>GPLGSEKIEKDNAFAFDLLQTTRKHVTEANVFISPLSVSMALNMTLNGAAGVTADEMKTALRETGYTMEDINEYSHSLREALLKVDPSTTIGMANSIWYKQGELVKEPFILANRTHYDAEVKAVDFSSPATLPAINGWCAQKTNDKITKILDYIPGNAFMYLINAVYFKGIWVTQFKKSDTKRAPFRKADGTTQEVNMMAQKSTFGYTTDECCQYLEMDYGNKAFSMIVMLPNEGQTTRDVIEQLDNKHWSMIIKGI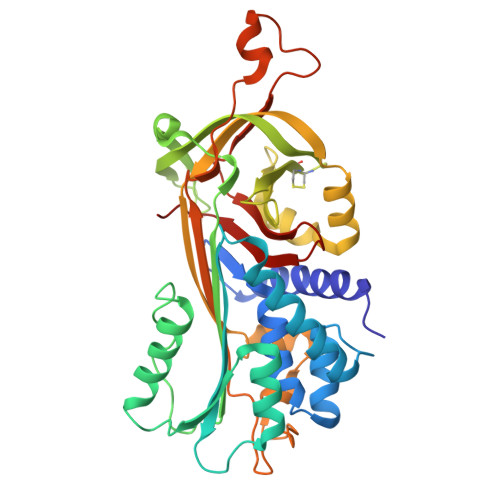RPTQVSLRMPRFKTECKYGLEKKILPEMGMNVPFTETADFPGITDAAIFISRVIHKTFVQVDEEGTEAAAVTAVEMVKTSSPSTTPINFHINKPFVFAIREKSTGVILFIGEIGEVKE[2x]> MEESKTPHVAIIPSPGMGHLIPLVEFAKRLVHLHGLTVTFVIAGEGPPSKAQRTVLDSLPSSISSVFLPPVDLTDLSSSTRIESRISLTVTRSNPELRKVFDSFVEGGRLPTALVVDLFGTDAFDVAVEFHVPPYIFYPTTANVLSFFLHLPKLDETVSCEFRELTEPLMLPGCVPVAGKDFLDPAQDRKDDAYKWLLHNTKRYKEAEGILVNTFFELEPNAIKALQEPGLDKPPVYPVGPLVNIGKQEAKQTEESECLKWLDNQPLGSVLYVSFGSGGTLTCEQLNELALGLADSEQRFLWVIRSPSGIANSSYFDSHSQTDPLTFLPPGFLERTKK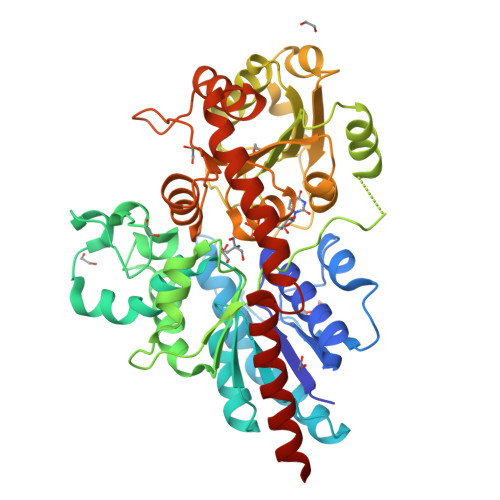RGFVIPFWAPQAQVLAHPSTGGFLTHCGWNSTLESVVSGIPLIAWPLYAEQKMNAVLLSEDIRAALRPRAGDDGLVRREEVARVVKGLMEGEEGKGVRNKMKELKEAACRVLKDDGTSTKALSLVALKWKAHKKELEQNGNH>[2x]DKLTLWTTPDPSPNCKIDQDKDSKLTFVLTKCGSQILANMSLLVVKGKFSMINNKVNGTDDYKKFTIKLLFDEKGVLLKDSSLDKEYWNYRSNNNNVGSAYEEAVGFMPSTTAYPKPPTPPTNPTTPLEKSQAKNKYVSNVYLGGQAGNPVATTVSFNKETGCTYSITFDFAWNKTYENVQFDSSFLTFSYIAQE

Here, we have sought to generate high-resolution crystallographic structures of the cellular interacting fiber-knob domains of species D adenoviruses HAdV-D26 and HAdV-D48. The fiber-knob is the receptor interacting domain of the fiber protein, one of three major capsid proteins along with the hexon and penton base, as shown schematically in Fig. 1a. We next calculated the amino acid variability at each position in the aligned adenoviral fiber-knob sequences, which revealed regions of broad conservation corresponding to β-strands which make up the main fold of the fiber-knob trimer. Each monomer interacts with two neighbouring copies to form a homotrimer with 3-fold symmetry and a highly stable interface. Analysis of the adenovirus loops reveals an intricate network of polar interactions which stabilise their three-dimensional structures.

The HAdV-D26K DG loop is most homologous to HAdV-B35K but incorporates a three amino acid insertion, while HAdV-D48K DG loop displays a differing and unique topology. The B-factors of the HAdV-D48K DG loop were observed to be polarised about the hairpin, with the outer face of the loop having higher B-factors compared to the inner face. This is likely the result of polar contacts formed between Ser-307, Gln-308, Ala-309, and Leu-304 with Asp-359 and Gln-357 of the opposing monomer stabilising the conformation of the DG loop. The proline-rich nature of this loop provides further rigidity. While loops which are less flexible and/or stabilised in a CAR inhibitory conformation, such as HAdV-D48K should result in a fiber-knob which is less able to bind CAR. This hypothesis fits the competition inhibition studies shown in Fig. 6c, which demonstrate that HAdV-D26K has an approximately ~15× lower affinity for CAR than HAdV-C5K, and HAdV-D48K has 500× lower affinity. The known CD46 utilising HAdV-B35K is seen to bind CD46 even at low concentration, while HAdV-D48K shows no interaction. Whilst we have not been able to model the interaction of HAdV-D26 or D48 with DSG2, due to the lack of an available high-resolution complexed structure at the time of writing, we investigated the interaction by SPR analysis. HAdV-B3 is the best studied DSG2 binding adenovirus and showed binding in the μM range when tested by SPR, however, no binding was observed when the same experiment was run with HAdV-D26K or HAdV-D48K. We demonstrate that HAdV-D26 and HAdV-D48 fiber-knob domains have a weak ability to bind CAR, and negligible CD46 interaction, suggesting that these viruses are unlikely to utilise these proteins as a primary receptor in vivo.> MKL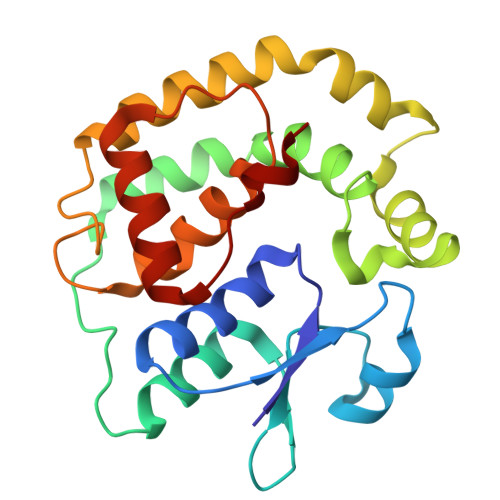YIYDHCPYCLKARMIFGLKNIPVELHVLLNDDAETPTRMVGQKQVPILQKDDSRYMPESMDIVHYVDKLDGKPLLTGKRSPAIEEWLRKVNGYANKLLLPRFAKSAFDEFSTPAARKYFVDKKEASAGNFADLLAHSDGLIKNISDDLRALDKLIVKPNAVNGELSEDDIQLFPLLRNLTLVAGINWPSRVADYRDNMAKQTQINLLSSMAI>[60x]MPWWYRRRSYNPWRRRNWFRRPRKTIYRRYRRRRRWVRRKPFYKRKIKRLNIVEWQPKSIRKCRIKGMLCLFQTTEDRLSYNFDMYEESIIPEKLPGGGGFSIKNISLYALYQEHIHAHNIFTHTNTDRPLARYTGCSLKFYQSKDIDYVVTYSTSLPLRSSMGMYNSMQPSIHLMQQNKLIVPSKQTQKRRKPYIKKHISPPTQMKSQWYFQHNIANIPLLMIRTTALTLDNYYIGSRQLSTNVTIHTLNTTYIQNRDWGDRNKTYYCQTLGTQRYFLYGTHSTAQNINDIKLQELIPLTNTQDYVQGFDWTEKDKHNITTYKEFLTKGAGNPFHAEWITAQNPVIHTANSPTQIEQIYTASTTTFQNKKLTDLPTPGYIFITPTVSLRYNPYKDLAERNKCYFVRSKINAHGWDPEQHQELINSDLPQWLLLFGYPDYIKRTQNFALVDTNYILVDHCPYTNPEKTPFIPLSTSFIEGRSPYSPSDTHEPDEEDQNRWYPCYQYQQESINSICLSGPGTPKIPKGITAEAKVKYSFNFKWGGDLPPMSTITNPTDQPTYVVPNNFNETTSLQNPTTRPEHFLYSFDERRGQLTEKATKRLLKDWETK

Anelloviruses are nonpathogenic viruses that comprise a major portion of the human virome. Our determination of the LY1 structure demonstrates that ORF1 encodes the capsid protein and that anelloviruses evolved a novel spike domain that extends around the 5-fold axis to form a crown structure. The particle, formed by 60 jelly roll domain-containing ANV capsid proteins, forms an icosahedral particle core from which spike domains extend to form a salient part of the particle surface. The base of the spike domain, the P1 subdomain, shares some sequence conservation between ANV strains while a hypervariable region, forming the P2 subdomain, is at the spike domain apex.

To generate a higher resolution structure, we generated an ORF1 polypeptide lacking the C-terminus (ΔC-Term) in human cells (Expi 293) and determined its structure. To generate an increased number of particles to permit higher resolution structure determination, we generated an ARM-containing ΔC-Term ORF1 construct (residues 1-609) for expression in Expi 293 cells. Western blot and Coomassie-stained sodium dodecyl-sulfate polyacrylamide gel electrophoresis (SDS-PAGE) analysis of the ΔC-Term ORF1 construct purified from mammalian cells showed a principal band consistent with the expected size. Despite containing the N-terminal ARM region, the ΔC-Term ORF1 formed symmetrical particles similar to the ΔARM fragments produced in insect cells, suggesting the presence of the ARM region does not hinder particle formation. We determined the cryo-EM structure of the virus-like particles formed by the insect cell-derived ΔARM fragment to 3.9 Å resolution from 6271 particles and of the mammalian cell-derived LY1 ΔC-Term ORF1 particle using cryo-EM to 2.69 Å resolution from 22,743 particles. Despite being generated in two different cell lines and the presence of the ARM region in the mammalian virus-like particle (which is not visible in the density, suggesting flexibility) the two protomer structures are very similar (1.179 Å root mean square deviation when aligned over residues 48–562). Particles from both expression systems adopt comparable folds, including an icosahedral particle core. Absent from both structures is the majority of the C-terminal region (in the higher resolution ΔC-Term particle, we see density up to residue 562). The portion of the C-terminus we can see extends from the jelly roll core toward the surface near the 2-fold axis between the spike domain crowns. The local resolution of P1 is only slightly lower than the jelly roll domain (~3–3.5 Å), while the resolution of P2 is within 4.5–5 Å.(TERT-BUTYLOXYCARBONYL)-ALANYL-ALANYL-AMINE | C11 H21 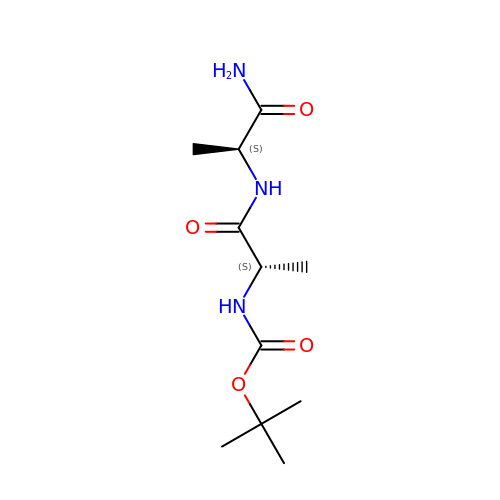N3 O4 | OAXZAMSRJZWMEV-BQBZGAKWSA-N>MFIQEPKKLIDTGEIGNASTGDILFDGGNKINSDFNAIYNAFGDQRKMAVANGTGADGQIIHATGYYQKHSITEYATPVKVGTRHDIDTSTVGVKVIIERGELGDCVEFINSNGSISVTNPLTIQAIDSIKGVSGNLVVTSPYSKVTLRCISSDNSTSVWNYSIESMFGQKESPAEGTWNISTSGSVDIPLFHRTEY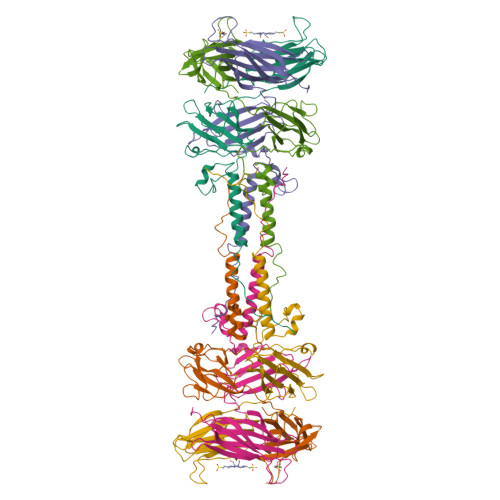NMAKLLVTCQSVDGRKIKTAEINILVDTVNSEVISSEYAVMRVGNETEEDEIANIAFSIKENYVTATISSSTVGMRAAVKVIATQKIGVAQ[2x]> MSFVDHPPDWLEEVGEGLREFLGLEAGPPKPKPNQQHQDQARGLVLPGYNYLGPGNGLDRGEPVNRADEVAREHDISYNEQLEAGDNPYLKYNHADAEFQEKLADDTSFGGNLGKAVFQAKKRVLEPFGLVEEGAKTAPTGKRIDDHFPKRKKARTEEDSKPSTSSDAEAGPSGSQQLQIPAQPASSLGADTMSAGGGGPLGDNNQGADGVGNASGDWHCDSTWMGDRVVTKSTRTWVLPSYNNHQYREIKSGSVDGSNANAYFGYSTPWGYFDFNRFHSHWSPRDWQRLINNYWGFRPRSLRVKIFNIQVKEVTVQDSTTTIANNLTSTVQVFTDDDYQLPYVVGNGTEGCLPAFPPQVFTLPQYGYATLNRDNTENPTERSSFFCLEYFPSKMLRTGNNFEFTYNFEEVPFHSSFAPSQNLFKLANPLVDQYLYRFVSTNNTGGVQFNKNLAGRYANTYKNWFPGPMGRTQGWNLGSGVNRASVSAFATTNRMELEGASYQVPPQPNGMTNNLQGSNTYALENTMIFNSQPANPGTTATYLEGNMLITSESETQPVNRVAYNVGGQMATNNQSSTTAPATGTYNLQEIVPGSVWMERDVYLQGPIWAKIPETGAHFHPSPAMGGFGLKHPPPMMLIKNTP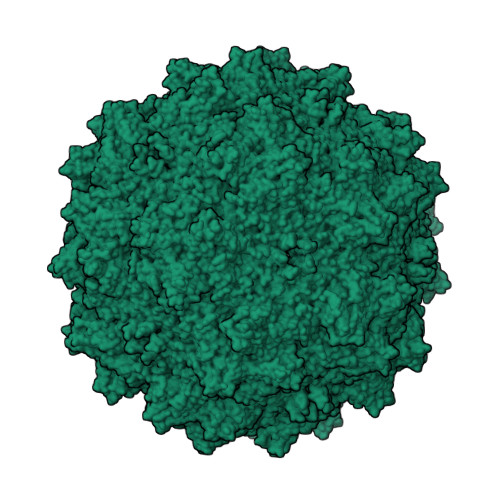VPGNITSFSDVPVSSFITQYSTGQVTVEMEWELKKENSKRWNPEIQYTNNYNDPQFVDFAPDSTGEYRTTRPIGTRYLTRPL>MAAESVRVAVRCRPFNQREKDLNTTLCVGMTPNVGQVNLNAPDGAAKDFTFDGAYFMDSTGEQIYNDIVFPLVENVIEGYNGTVFAYGQTGSGKTFSMQGIETIPAQRGVIPRAFDHIFTATATTENVKFLVHCSYLEIYNEEVRDLLGADNKQKLEIKEQPDRGVYVAGLSMHVCHDVPACKELMTRGFNNRHVGATLMNKDSSRSHSIFTVYVEGMTETGSIRMGKLNLVDLAGSERQSKTGATGDRLKEATKINLSLSALGNVISALVDGKSKHIPYRDSKLTRLLQDSLGGNTKTIMIACVSPSSDNYDETLSTLRYANRAKNIKNKPTINEDPLEHHHHHH[2x]

OSM‐3 belongs to the homodimeric kinesin‐2 subfamily and is the Caenorhabditis elegans homologue of human KIF17. Similar to KIF17, OSM‐3 is involved in intraflagellar transport in the distal part of the cilium, and both proteins are autoinhibited at the resting state. The OSM‐3 motor domain shows the typical kinesin fold, with a central eight‐stranded β‐sheet surrounded by 3 α‐helices on either side. We have determined the structure of the motor domain of OSM‐3 either bound to ADP or to AMPPNP, or devoid of a nucleotide.

OSM‐3 was incubated with apyrase in the presence of this stable ATP analog and crystals diffracting X‐rays up to 1.9 Å were obtained. The structure was solved by molecular replacement using ADP‐OSM‐3 as a search model, with two very similar molecules in the asymmetric unit (rmsd 0.50 Å; 335 Cαs compared). Electron density maps clearly indicate the presence of AMPPNP in the nucleotide‐binding site. In particular, the Switch 2‐L11‐α4 region is fully ordered, with a short helical segment formed in L11 and α4 extended at its N‐terminal region by about 2.5 turns compared to ADP‐OSM‐3. The L9‐Switch 1 region also becomes ordered and adopts a hairpin conformation. Therefore, the nucleotide‐binding site of AMPPNP‐OSM‐3 is in a ‘closed’ conformation. Much of this is due to a ~ 15° rotation of α4 and to a ~ 2 Å translation of α5, two helices involved in the interaction with microtubules. In particular, two water molecules in the OSM‐3 nucleotide‐binding site overlap with W1 and W2 of Eg5. The residues that are within hydrogen bond distance to these water molecules belong to the Switch 1 (Ser204 (carbonyl oxygen) and Arg205 in OSM‐3) and Switch 2 (Gly235 and Glu237) motifs. Further comparisons indicate that, similar to isolated kinesin‐4 and kinesin‐5, AMPPNP‐OSM‐3 adopts the structure of tubulin‐bound or microtubule‐bound ATP‐like kinesin‐1, kinesin‐6, kinesin‐8, and kinesin‐13, suggesting that AMPPNP‐OSM‐3 displays the microtubule‐bound ATP conformation of OSM‐3.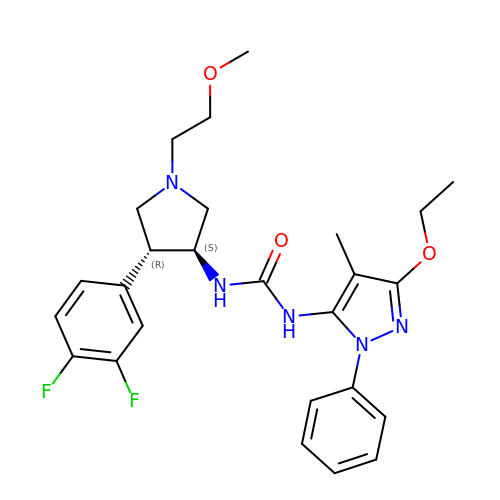1-[(3S,4R)-4-[3,4-bis(fluoranyl)phenyl]-1-(2-methoxyethyl)pyrrolidin-3-yl]-3-(5-ethoxy-4-methyl-2-phenyl-pyrazol-3-yl)urea | C26 H31 F2 N5 O3 | SQGLEZDWHPDRDX-NZQKXSOJSA-N4-({(3R)-7-(5-formylfuran-2-yl)-4-[(4-methoxyphenyl)sulfonyl]-1-[(1-methyl-1H-imidazol-5-yl)methyl]-2,3,4,5-tetrahydro-1H-1,4-benzodiazepin-3-yl}methyl)phenyl 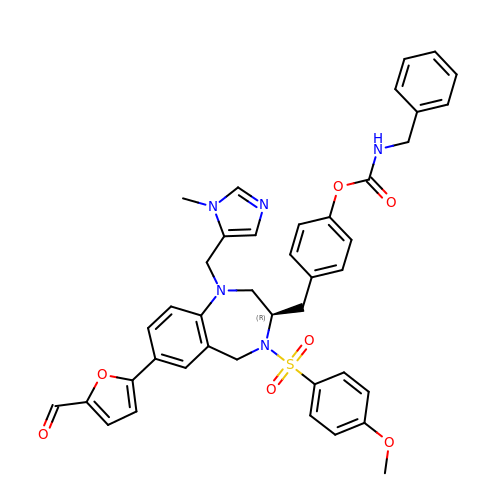benzylcarbamate | C41 H39 N5 O7 S | GAZNDTRYZUUOKB-MGBGTMOVSA-N> MLRGWHPNSSAMQVGMRHITIGGRHSRGGFRQPLGKHPQVKQGTVEGVPRRIPGTTKVTYTNKKGRTFSFSVPVSELTHPQVTLESAAGTWREMDTSFCELGDIEDDMPSPVDECLRGGSSLDKRLIQEVRERFVSFCREYVLMDTSGMKSTILSTELNAGPDYEHYDRRLRRKRHWLAIRHRFEDVRYVIWPDVVEETARGDSAQADVSLTNPSLTAGEMLEALLWLDAASTFCVRKVHPSDLGDKSEFLPLDLQREVEVVACHARRDLDFFDPSATSLEQFTACAALCVNHRVPFSLFFPAQDVC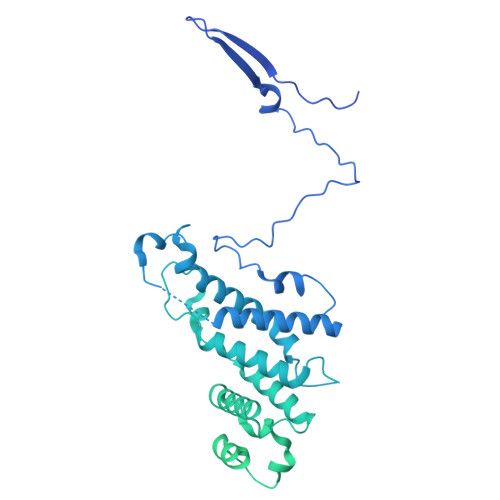GDASVSTGQCIVANAPSPHTALGAVRIMALISEGSGSDIGKTIMFSDAFGAVTRFGILRGLSRVMSVEAFGCKDALENVNESELCIILHFCAEVREQNAAFFRRYEASEEDSDPQQVSFLAKYQQLSQIALARCKRLLYHPDSPRAQVMSEDGYIPLVELQRHAEGTNKAALIHYNLGIRSAQGMRRVALGAQSSARLAELVSRLEEASARVSGNTLVNDLVHHLSHKAAAGKMSLTLREVNTLLPLLSRMRRESPNGALDARFDRVFNAIDTAIGAAMRHNCTLDELLDLAEGLAACEMVPSALKQVEMVLIRSVMMHECSPMHLRRMLQAMFTLMRTSVPQVLLQSVASRVADYIKEASHMDSSSSNGGGDEKVKNHEECEQLLELLVVLGKCGYGALPGLVTIYWEAQLIDSMQLNPRLRCSYASLLASAAFALKKHDKRAWEGLADESHRLFMEYTRCNKENDIGRFAECVTGLAVLTQIKDNTNSSDVAFLKEYLSATSLELKSCEVIRVQELTDLLGRTLEWSEALGVVAPDVVIQLEKALFVMLENVSHTAPGVGIPDELVTAACCLVDMSSASLELRKAAAGVVGGAIVHAEEALETLRSGAPTQVRPGHSFDVAALASAERENVYKNSILQYCAALQRSGMSTHVEELWS> AIPWGGNLEEVLEELEMALLAADVGLSATEEILQEVRASGRKDLKEAVKEKLVGMLEPDERRATLRKLGFNPQKPKPVEPKGRVVLVVGVNGVGKTTTIAKLGRYYQNLGKKVMFCAGDTFRAAGGTQLSEWGKRLSIPVIQGPEGTDPAALAYDAVQA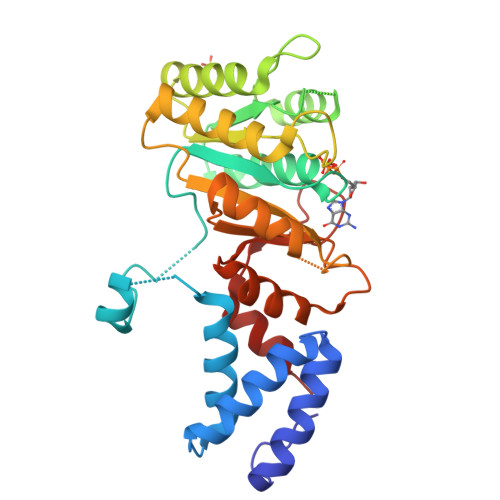MKARGYDLLFVDTAGRLHTKHNLMEELKKVKRAIAKADPEEPKEVWLVLDAVTGQNGLEQAKKFHEAVGLTGVIVTKLDGTAKGGVLIPIVRTLKVPIKFVGVGEGPDDLQPFDPEAFVEALLED>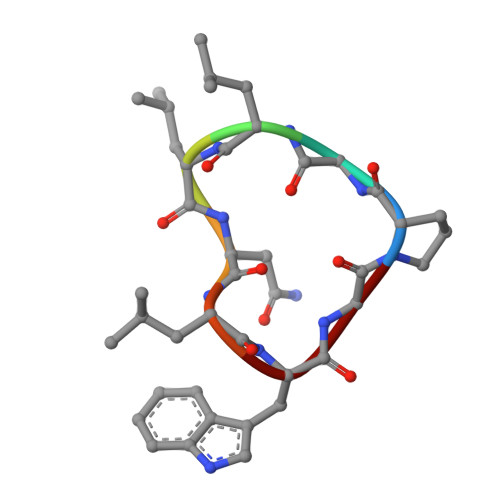 PGLLNLWG> MAHHHHHHMSTSSRCLVRGSVNIDEFFHLPHIVRPGETISSTGLTKRAGGKGANQAFAVARAGGQVELDGAIGDDGIWVKEMLESAGVGTDKLKIVKDEVTGRAVIQSAADGENSIVLHAGANYYLPSPTPTTSLATYTHLLVQNEVPLSS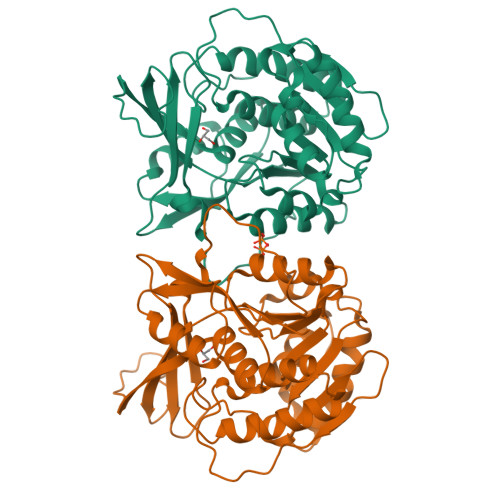TLAYLTAAGQSSPPLTSVFNPSPMLTPAQLREFPWKHLSWLIVNEGELGDLLLAFGSSANPGEAKEDELQAKASAGILELHENDYFSKNVGIICTLGAKGILCYEPGKEVGYLPAAKLQNPVKDTTGAGDCFAGYFVAGLMSGKSLQDALKTCLVACGICVENEGAMESVPTLNAVKERLA>MKGTIVGTWIKTLRDLYGNDVVDESLKSVGWEPDRVITPLEDIDDDEVRRIFAKVSEKTGKNVNEIWREVGRQNIKTFSEWFPSYFAGRRLVNFLMMMDEVHLQLTKMIKGATPPRLIAKPVAKDAIEMEYVSKRKMYDYFLGLIEGSSKFFK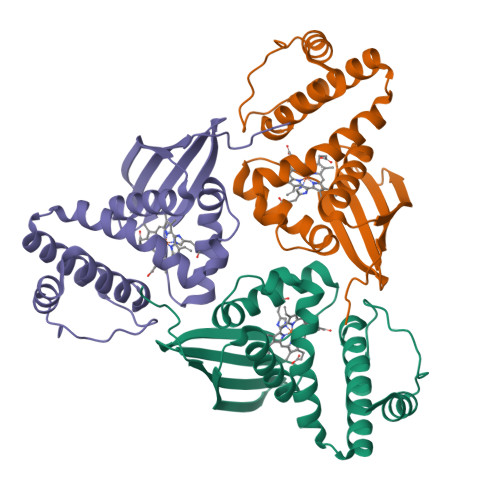EEISVEEVERGEKDGFSRLKVRIKFKNPVFEYKKN[6x]2-[[4-[4-[(2-carboxyphenyl)carbamoyl]phenoxy]phenyl]carbonylamino]benzoic 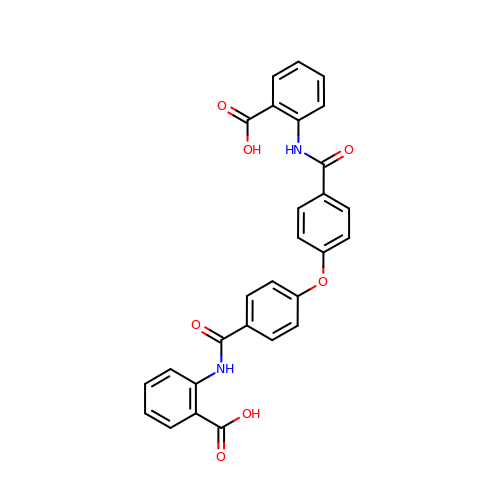acid | C28 H20 N2 O7 | UIRNMCRFFYWCBB-UHFFFAOYSA-N> MADRVDARRATWWSVVNILVIVYALIPVLWILSLSLKPTSSVKDGKLIPTEITFANYKAIFSGDAFTSALFNSIGIGLITTIIAVVIGGMAAYAVARLQFPGKQLLIGVALLIAMFPHISLVTPIFNMWRGIGLFDTWPGLIIPYITFALPLAIYTLSAFFREIPWDLEKAAKMDGATPAQAFRKVIAPLAAPGIVTAAILVFIFAWNDLLLALSLTATQRAITAPVAIANFTGSSQFEEPTGSIAAGAMVITIPIIIFVLIFQRRIVAGLTS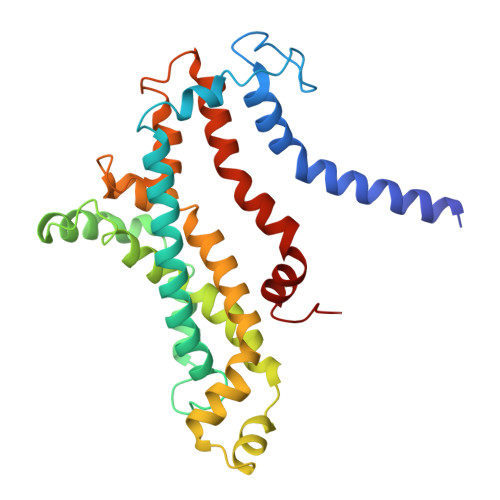GAVKG>[2x]MARDARKRTS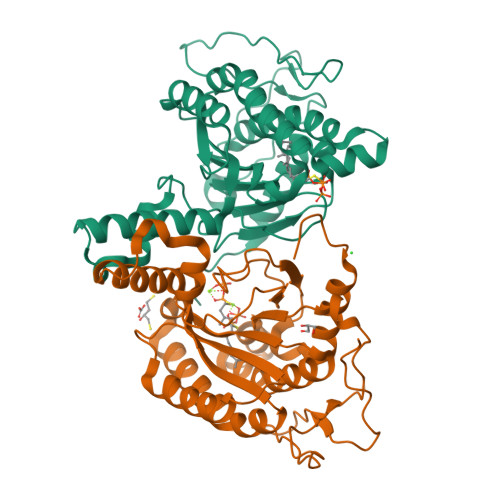SNFPQLPPAPDDYPTFPDTSTWPVVFPELPAAPYGGPCRPPQHTSKAAAPRIPADRLPNHVAIVMDGNGRWATQRGLARTEGHKMGEAVVIDIACGAIELGIKWLSLYAFSTENWKRSPEEVRFLMGFNRDVVRRRRDTLKKLGVRIRWVGSRPRLWRSVINELAVAEEMTKSNDVITINYCVNYGGRTEITEATREIAREVAAGRLNPERITESTIARHLQRPDIPDVDLFLRTSGEQRSSNFMLWQAAYAEYIFQDKLWPDYDRRDLWAACEEYASRTRRFGSA>MDPPARKEKTKVKESVSRVEKAKQKSAQQELKQRQRAEIYALNRVMTELEQQQFDEFCKQMQPPGE[2x];>MDEATWERMWKHVAKIHPDGEKVAQRIRGATDLPKIPIPSVPTFQPSTPVPERLEAVQRYIRELQYNHTGTQFFEIKKSRPLTGLMDLAKEMTKEALPIKCLEAVILGIYLTNSMPTLERFPISFKTYFSGNYFRHIVLGVNFAGRYGALGMSRREDLMYKPPAFRTLSELVLDFEAAYGRCWHVLKKVKLGQSVSHDPHSVEQIEWKHSVLDVERLGRDDF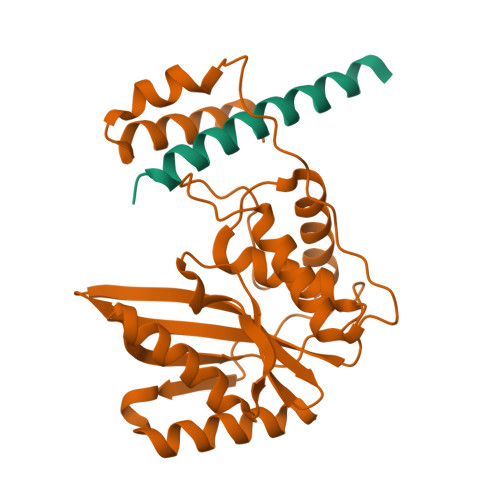RKELERHARDMRLKIG[2x]Here we report that histones are major chromatin components in the bacteria Bdellovibrio bacteriovorus and Leptospira interrogans. Crystal structures (<2.0 Å) of the B. bacteriovorus histone (Bd0055) dimer and the histone–DNA complex confirm conserved histone-fold topology but indicate a distinct DNA-binding mode. Unlike known histones in eukaryotes, archaea and viruses, Bd0055 binds DNA end-on, forming a sheath of dimers encasing straight DNA rather than wrapping DNA around their outer surface. The bacterial histone Bd0055 from B. bacteriovorus HD100 is structurally similar to its archaeal and eukaryotic homologues but, rather than wrapping DNA around its outer surface, binds DNA edge-on and oligomerizes to form a dense nucleohistone fibre that completely encases DNA in vitro.

To understand how Bd0055 binds DNA, we solved the crystal structure of Bd0055 in complex with a 35 bp DNA fragment. This structure shows that Bd0055 contacts the DNA with only one L1-L2 binding interface across the minor groove. The molecular details of this edge-on interaction are very similar to those observed for other known histones. It employs the L1-L2 motif that is conserved across the domains of life, although the sprocket arginine that reaches into the minor groove in nearly all other histone–DNA complexes is missing. Surprisingly, rather than the DNA bending around the positively charged histone surface, the DNA maintains a straight trajectory. Additional histone dimers bind the next two phosphates through L1-L2 interfaces engaged in identical interactions but flipped by 180 degrees. The filament is stabilized through protein–protein interactions between histone dimers that involve the basic DNA-binding ridge and the acidic underside of histone dimers 1 and 5, and through exchanging N-terminal tails between dimers 1 and 4. This nucleohistone filament, which is characterized by a histone to DNA ratio of 1 histone dimer per 2.5 bp, reverses known histone convention by completely protecting straight DNA from the solvent. The crystal lattice we observed suggests the possibility that bacterial histones might generate higher-order fibre packing through the interaction of histones on adjacent nucleohistone filaments.

>[2x]MAEVLVVTSKVKKLIKEKGQMNTSAETIDVLSKAIEQLCLKGVESAKADGRKTVMARDIVIDHL>MNHYEVLVLGGGSGGITMAARMKRKVGAENVAIVEPSERHFYQPIWTLVGAGAKQLSSSGRPTASVIPSGVEWIKARVTELNPDKNCIHTDDDEKISYRYLIIALGIQLDYEKIKGLPEGFAHPKIGSNYSVKTVEKTWKALQDFKEGNAIFTFPNTPVKCAGAPQKIMYLSEAYFRKTGKRSKANIIFNTSLGAIFGVKKYADALQEIIQERNLTVNYKKNLIEVRADKQEAVFENLDKPGETQVISYEMLHVTPPMSPPDVLKTSPVADAAGWVDVDKETLQHRRYPNVFGIGDCTNLPTSKTAAAVAAQSGILDRTISVIMKNQTPTKKYDGYTSCPLVTGYNRVILAEFDYKAEPLETFPFDQSKERLSMYLMKADLMPFLYWNMMLRGYWGGPA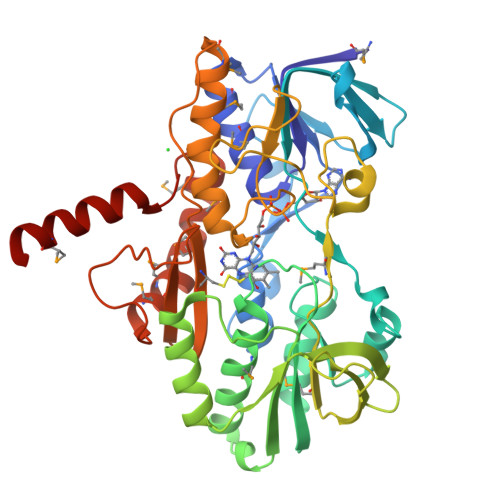FLRKLFHLGMSLEHH[4x]> GAMAMSDLPIEFTELVDLMSLGISPQFLDFRSTTFESDHFVTVRETKDGTNSVAIVDLAKGNEVTRKNMGGDSAIMHPSQMVISVRANGTIVQIFNLETKSKLKSFTLDEPVIFWRWLSETTLGFVTARSILTSNVFDGNVNAKPQLLTLRHANLNNTQIINFVANKNLDWFAVVGILQENGRIAGRIQLFSKQRNISQAIDGHVAIFTNILLEGNGSTPVQVFVTGNRNATTGAGELRIIEIDHDASLPSQYQKETTDIFFPPDATNDFPIAVQVSEKYGIIYLLTKYGFIHLYELETGTNLFVNRITAESVFTAAPY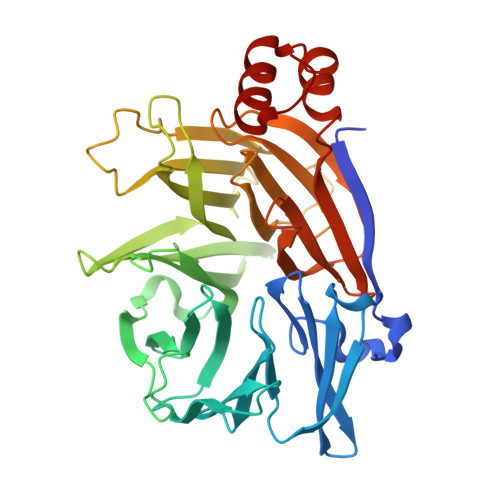NHENGIACINKKGQVLAVEISTSQIVPYILNKLSNVALALIVATRGGLPGADDL> HHHHHHIEGRGAYVLDDSDGLGREFDGIGAVSGGGATSRLLVNYPEPYRSEILDYLFKPNFGASLHILKVEIGGDGQTTDGTEPSHMHYELDENYFRGYEWWLMKEAKKRNPDIILMGLPWSFPGWLGKGFSWPYVNLQLTAYYVVRWILGAKHYHDLDIDYIGIWNERPFDANYIKELRKMLDYQGLQRVRIIASDNLWEPISSSLLLDQELWKVVDVIGAHYPGTYTVWNAKMSGKKLWSSEDFSTINSNVGAGCWSRILNQNYINGNMTSTIAWNLVASYYEELPYGRSGLMTAQEPWSGHYVVASPIWVSAHTTQFTQPGWYYLKTVGHLEKGGSYVALTDGLGNLTIIIETMSHQHSMCIRPYLPYYNVSHQLATFTL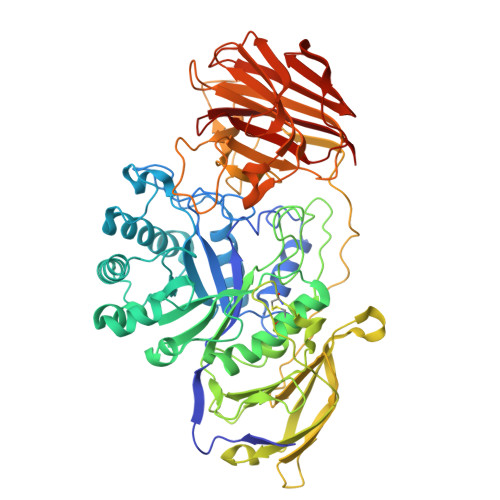KGSLREIQELQVWYTKLGTPQQRLHFKQLDTLWLLDGSGSFTLELEEDEIFTLTTLTTGRKGSYPPPPSSKPFPTNYKDDFNVEYPLFSEAPNFADQTGVFEYYMNNEDREHRFTLRQVLNQRPITWAADASSTISVIGDHHWTNMTVQCDVYIETPRSGGVFIAGRVNKGGILIRSATGVFFWIFANGSYRVTADLGGWITYASGHADVTAKRWYTLTLGIKGYFAFGMLNGTILWKNVRVKYPGHGWAAIGTHTFEFAQFDNFRVEAAR(1R,2R,3R)-5-[(E)-2-[(1R,3aS,7aR)-7a-methyl-1-[(2R)-6-methyl-6-oxidanyl-heptan-2-yl]-1,2,3,3a,6,7-hexahydroinden-4-yl]ethenyl]-2-(3-oxidanylpropyl)cyclohex-4-ene-1,3-diol 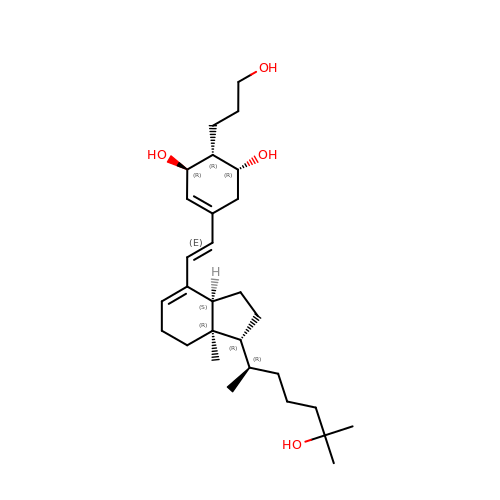| C29 H48 O4 | FSKKMLBYNCANGG-LIDHDOQTSA-N> EPVNLIFCYTILQMKVAERIMAQHPGERFYVVLMSENRNEKYDYYFNQIKDKAEWAYFFHLPYGLNKSFNFIPTMAELKVKAMLLPKVKRIYLASLEKVSIAAFLSTYPDAEIKTFDDGTINLIQSSSYLGDEFSVNGTIKRNFARMMIGDWSIAKTRNASDEHYTIFKGLKNIMDDGRRKMTYLPLFDASELKAGDETGGTVRILLGSPDKEMKEISEKAAKNFNIQYVAPHPRQTYGLSGVTTLNS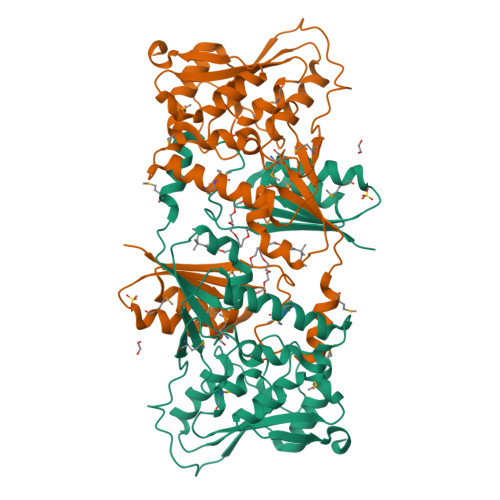PYVIEDYILREIKKNPHTRYEIYTFFSGAALTMKDFPNVHVYALKPASLPEDYWLKPVYALFTQSGIPILTFDDKLVPR>TSLFTTADHYHTPLGPDGTPHAFFEALRDEAETTPIGWSEAYGGHWVVAGYKEIQAVIQNTKAFSNKGVTFPRYETGEFELMMAGQDDPVHKKYRQLVAKPFSPEATDLFTEQLRQSTNDLIDARIELGEGDAATWLANEIPARLTAILLGLPPEDGDTYRRWVWAITHVENPEEGAEIFAELVAHARTLIAERRTNPGNDIMSRVIMSKIDGESLSEDDLIGFFTILLLGGIDATARFLSSVFWRLAWDIELRRRL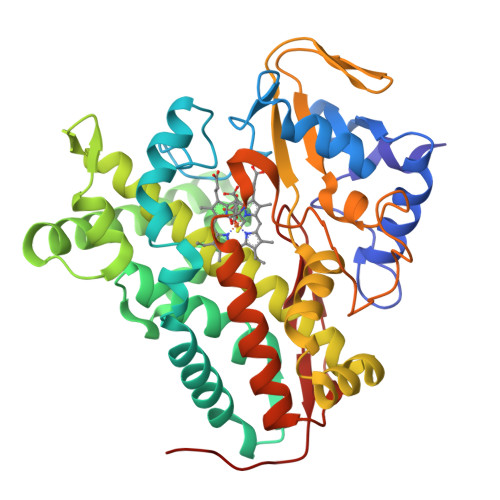IAHPELIPNAVDELLRFYGPAMVGRLVTQEVTVGDITMKPGQTAMLWFPIASRDRSAFDSPDNIVIERTPNRHLSLGHGIHRCLGAHLIRVEARVAITEFLKRIPEFSLDPNKECEWLMGQVAGMLHVPIIFPKGKRLSE[2x]> GSNS;> MSSNSLALKGRSDAYTQVDNFLHAYARGGDELVNGHPSYTVDQAAEQILREQASWQKAPGDSVLTLSYSFLTKPNDFFNTPWKYVSDIYSLG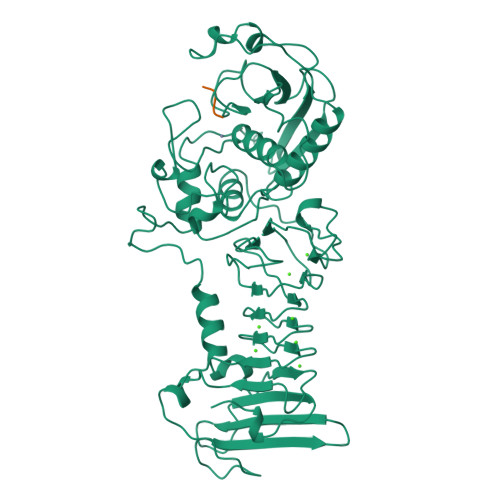KFSAFSAQQQAQAKLSLQSWSDVTNIHFVDAGQGDQGDLTFGNFSSSVGGAAFAFLPDVPDALKGQSWYLINSSYSANVNPANGNYGRQTLTHEIGHTLGLSHPGDYNAGEGDPTYADATYAEDTRAYSVMSYWEEQNTGQDFKGAYSSAPLLDDIAAIQKLYGANLTTRTGDTVYGFNSNTERDFYSATSSSSKLVFSVWDAGGNDTLDFSGFSQNQKINLNEKALSDVGGLKGNVSIAAGVTVENAIGGSGSDLLIGNDVANVLKGGAGNDILYGGLGADQLWGGAGADTFVYGDIAESSAAAPDTLRDFVSGQDKIDLSGLDAFVNGGLVLQYVDAFAGKAGQAILSYDAASKAGSLAIDFSGDAHADFAINLIGQATQADIVV> MGVPALFRWLSRKYPKIISPVIQDEDVDIDGESRPTRYEDPNPNGELDNLYLDMNGIVHPCSHPEHKPVPETEDEMMLDVFAYTENVIMMARPRKVIYIAVDGVAPRAKMNQQRSRRFRSAQDAKDANEKKAAELKEMEKKGEIIDDAIKNKKTWDSNAITPGTPFMHRLADSLRYWAAYKLTTDPGWSGIEVIISDASVPGEGEHKIMSYVRSLRSSPKHDPNTTHCIYGLAAALIFLGLATHEPHFKILREDVFAQDKKSYSLQDQLRMTDIERQELKDKKTPFLWLHLNILREYLQIELNVPGLSFPFDLEKSIDDWVFICFFCGNDFLPHLPSLDVRDNSITTLVTIWKQILPTMKGYLTTDGYLNLPAVERLLAELAKKEDYIFRKRYEDEKRSLENQKRRKLAQEQSSARSQNAPNISTGKDKAPLTPNQNIPLYTTSGESVGIKMTDSEMVNNSALITKANEANKSIAELLKQNLQNEINKKRKISNEEQEVVKESVEEVVEEEDDVLVTSDPEDSSTEILIPKNEEIRLWEPGYRKRYYETKFHTKDPQKVKKIARNMVQKYIEGVSWVLLYYYQGCPSWNWYYPYHYAPFAADFVNLSELKIEFVEGTPFRPYEQLMSVLPAASSHNLPDVFRSLMSDANSEIIDFYPEEFPLDMNGKKVIWQAIPLLPFIDENRLLKAVQSKYDQLTEDEKFRNTNRSEILVLGRSHSHYPTLVKELYEEGKDSYEFQVDSSGVSGVAIKLQSFDRSGVLRLPVKQLEGYRHYPDISNRDFLMVEFKQLPKSHAKSMILSGLIPHLRRLTQEDKDSILYGGTNFYGRNRFSPEENADFKQYIGPHGKSQYLPRQGGYKAFIQIHSDEAKGHRHGIYHGGSHTETEFRRGGGYHQHGNRGGRGGYQGNQ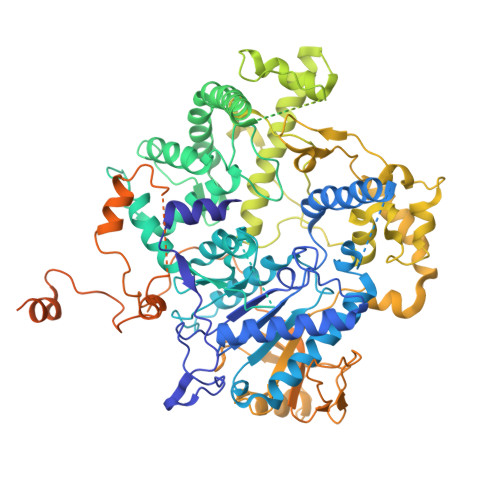GYQANSGGYQNSYQGSYQGGYRGGYQGGSQGRYQAGYQSGYQGGYQGEYKNGYQGGYQGNQGNQGYNRQTYNASKSGTLPMKRRHNSGPSSGLEVLFQ(2S,3S)-3-methyl-aspartic 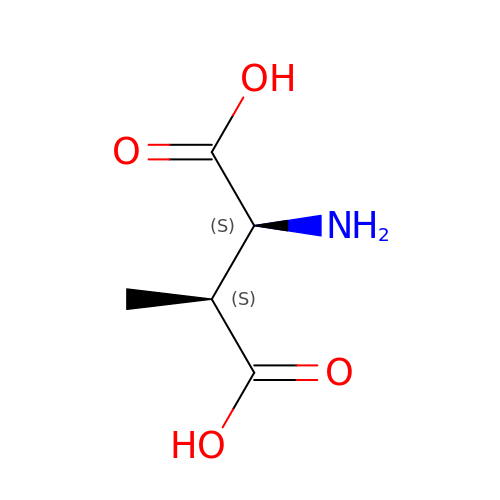acid | C5 H9 N O4 | LXRUAYBIUSUULX-HRFVKAFMSA-N> QPIFLNVLEA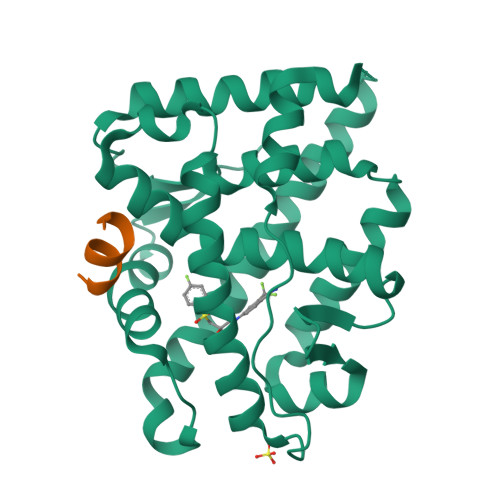IEPGVVCAGHDNNQPDSFAALLSSLNELGERQLVHVVKWAKALPGFRNLHVDDQMAVIQYSLMGLMVFAMGWRSFTNVNSAMLYFAPDLVFNEYRMHKSRMYSQCVRMRHLSQEFGWLQITPQEFLCMKALLLFSIIPVDGLKNQKFFDELRMNYIKELDRIIACKRKNPTSCSRRFYQLTKLLDSVQPIARELHQFTFDLLIKSHMVSVDFPEMMAEIISVQVPKILSGKVKPIYFHTQ;> KTRYIFDLFYKRKAY> AKLLEQIEKWAAETPDQTAFVWRDAKITYKQLKEDSDALAHWISSEYPDDRSPIMVYGHMQPEMIINFLGCVKAGHAYIPVDLSIPADRVQRIAENSGAKLLLSATAVTVTDLPVRIVSEDNLKDIFFTHKGNTPNPEHAVKGDENFYIIYTSGSTGNPKGVQITYNCLVSFTKWAVEDFNLQTGQVFLNQAPFSFDLSVMDIYPSLVTGGTLWAIDKDMIARPKDLFASLEQSDIQVWTSTPSFAEMCLMEASFSESMLPNMKTFLFCGEVLPNEVARKLIERFPKATIMNTYGPTEATVAVTGIHVTEEVLDQYKSLPVGYCKSDCRLLIMKEDGTIAPDGEKGEIVIVGPSVSVGYLGSPELTEKAF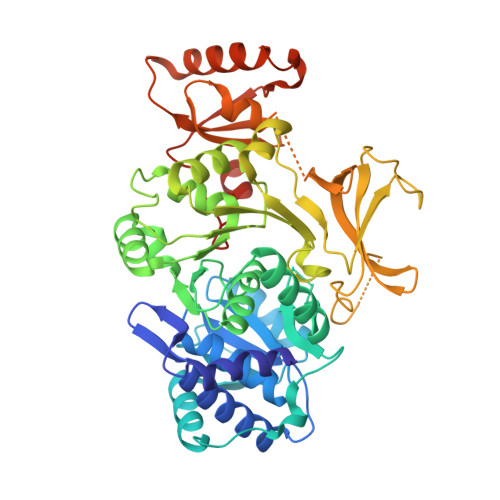TMIDGERAYKTGDAGYVENGLLFYNGRLDFQIKLHGYRMELEEIEHHLRACSYVEGAVIVPIKKGEKYDYLLAVVVPGEHSFEKEFKLTSAIKKELNERLPNYMIPRKFMYQSSIPMTPNGKVDRKKLLSEVTALEHHHHHH6-(2-{5-[2-(2-amino-6-methylpyridin-4-yl)ethyl]pyridin-3-yl}ethyl)-4-methylpyridin-2-amine 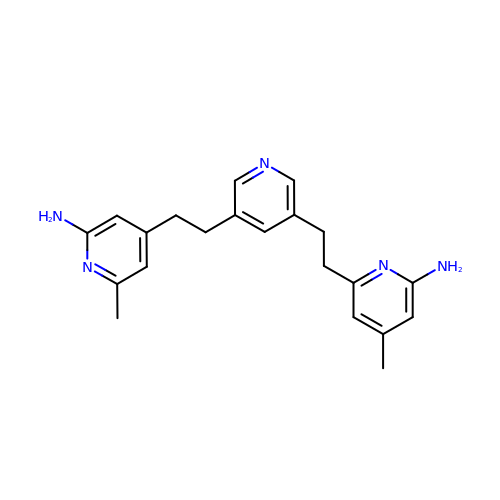| C21 H25 N5 | RDXKSGCNYFTVRW-UHFFFAOYSA-N> MGKLIRLELFNFKSYKGHHTLLFGDSYFTSIIGPNGSGKSNSM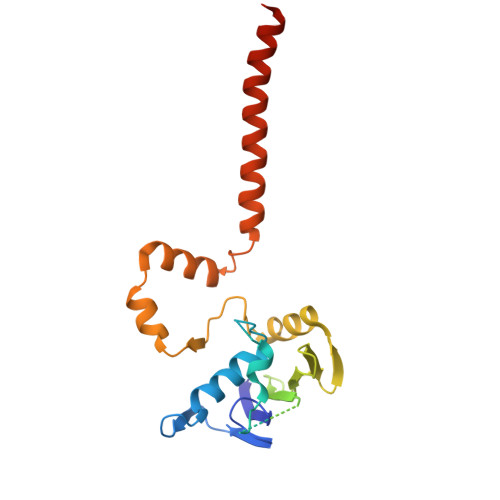DAISFVLGIKSSHLRSSNLRDLIYRGRVMKTSKIQDDGTTAPATNGDVNGYENGDAGDDEDTSQRTSRNDPKTAWVMAVYEDDAGELHRWKRTITANGTSEYRINDRVVNAQQYNEALEKENILIKARNFLVFQGDVEAIASQSPQDLTRLIEQISGSLEYKEEYERLEEEVRQATEEQAYKLQRRRAANSEIKQYMEQ> MVSLTKRCIAEFIGTFILVFFGAGSAAVTLMIASGGTSPNPFNIGIGLLGGLGDWVAIGLAFGFAIAASIYALGNISGCHINPAVTIGLWSVKKFPGREVVPYIIAQLLGAAFGSFIFLQCAGIGAATVGGLGATAPFPGISYWQAMLAEVVGTFLLMITIMGIAVDERAPKGFAGIIIGLTVAGIITTLGNISGSSLN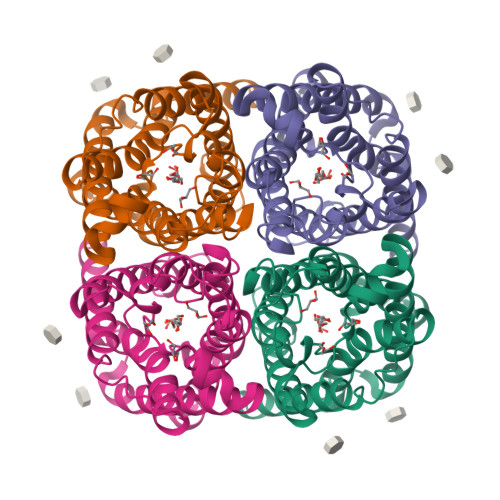PARTFGPYLNDMIFAGTDLWNYYSIYVIGPIVGAVLAALTYQYLTSE1-[[(1~{R})-2-[(5-chloranylpyridin-2-yl)methyl]-1-(4-chlorophenyl)-7-fluoranyl-3-oxidanylidene-5-(2-oxidanylpropan-2-yl)isoindol-1-yl]oxymethyl]cyclopropane-1-carboxamide 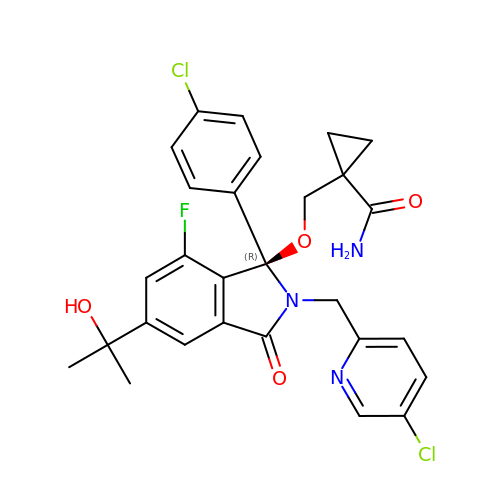| C28 H26 Cl2 F N3 O4 | QEBHYSMAGWDGTO-MUUNZHRXSA-N> MGSSHHHHHHSSGRENLYFQGHMEVHEEQVSAPVTGDATAKYLLQYILSARGICHENALILALMRLETDASTLNTEWSIQ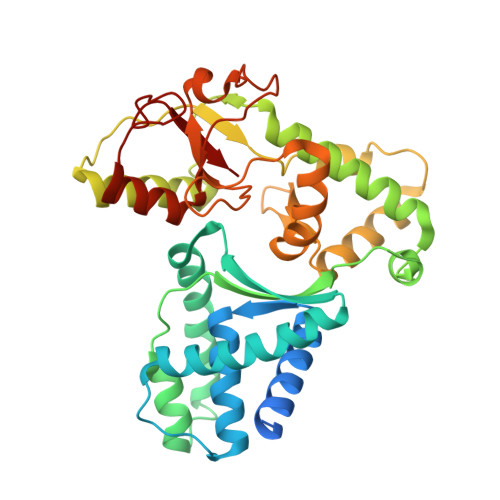QWVDKLNDYINAINVKLNLLGYKIIRINHGIGRNAVTLKAKQNFESFEDNTAIRAHNNDYAVLQSIVLPESNRFFVYVNLASTEETKLATRFNQNEIEFMKWAIEQFMISGETIVEGPALETSIIVKEVNRILVAATGDSNLAKWRKFSTFTVGSTNLFQFQELTATDIEDLLLRLCELKWFYRTQEGKFGIDLRCIAELEEYLTSMYNLNTCQNCHKLAIQGVRCGNESCREENEETGENSLSQIWHVDCFKHYITHVSKNCDRCGSSLITEGVYVI> MATEFTPSVYSLVSKPLPSNSRPSATLDEQAETEDLISQLFDLTADPNALVSEHGKRYSGLRKQEHTQFLASSFFQLPGKFVSLDASRPWLVFWTVHSLDLLGVALDQGTKDRVVSTLLHFLSPKGGFGGGPANSQIPHLLPTYASVCSLAIAGNDSSTGGWKDLAAARQSIYEFFMRCKRPDGGFVVCEGGEVDVRGTYCLLVVATLLDIITPELLHNVDKFVSACQTYEGGFACASFPFPSVVPSTSAFPTSEPSCRVSMAEAHGGYTSCSLNSHFLLTSVPLPSFPLSIDANAALRWTVLQQGEPIEGGGFRGRTNKLVDGCYSWWVGGGAPVAEELVRREKSRKVKKSRIEVFEEEKEGDWEDVPPIPPIFNRVALQEFTLVAAQQDPGSTGGLRDKPGKRPDQYHTCNNLSGLSIAQHKMSHSPS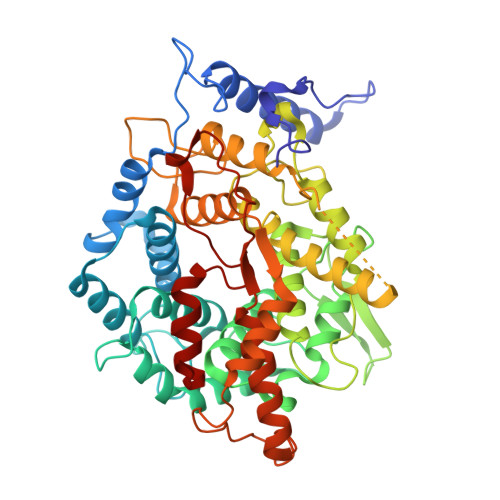TVSSNRLKFDASKGLPAVKPVAPGGGWKNEDERQNARREIWANALGWIEEEGGEIIVGGKDNRINTTTPVFNILGLRLKPFINYFYCQEN> GSHMRSRRVDVMDVMNRLILAMDLMNRDDALRVTGEVREYIDTVKIGYPLVLSEGMDIIAEFRKRFGCRIIADFAVADIPETNEKICRATFKAGADAIIVHGFPGADSVRACLNVAEEMGREVFLLTEMSHPGAEMFIQGAADEIARMGVDLGVKNYVGPSTRPERLSRLREIIGQDSFLISPGVGAQGGDPGET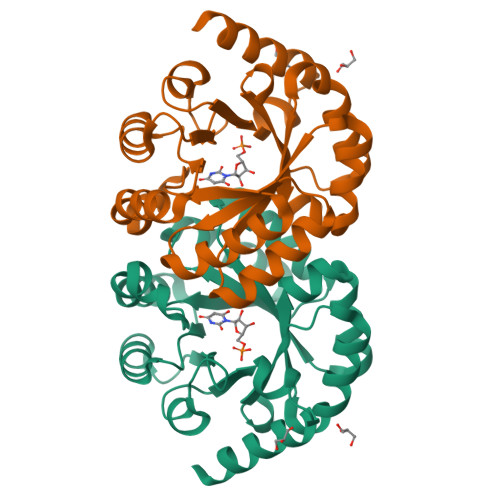LRFADAIIVGRSIYLADNPAAAAAGIIESIKDLRIPEDPAANKARKEAELAAATAEQ>MAGRRKQRRSRAPRRKRTTGRKTLKRKADSRATPAKSTRKRTKTVSGAAKHHAVRVKPFSNATTQPKIPDGLLTSSLSRRLQNVVGVRNGNSPSVHAGSDVMHVVIAPTLGVPVMIANSAEGVLKRPGLSQESSFIGFPGQTVGFENLIESTGVPTWPPTIPTGQKLENKGGFVLWRIISQGLRIDLANSDEENDGWFEACRFNWRNVPRDVCMTPLDGSTTTNSIGIAPNPLWLEEVGYGMAMVEQPGYKSGLLKDIKKAEFMLHPRTTTHDPTLIDPFEYGGSMTSSGGIDNVYYPSDNVSGNAVRFRDMGVDQNMDWIYIRLHCRPNNGTSSLGSNFLFNVIQN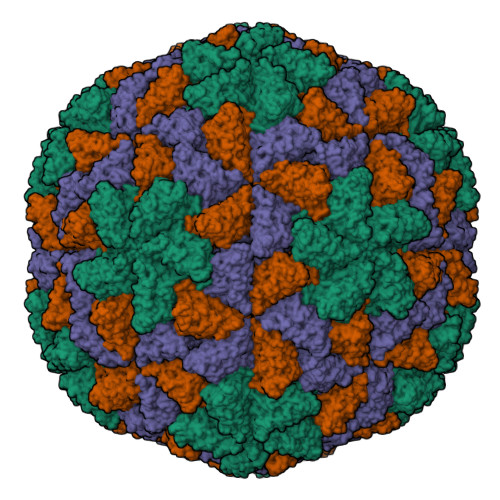VEVAFNPSSDFAAFQTINKADTKTKMVADGLNNNPDVFNGRRK[3x]>MLQVHRTGLGRLGVSLSKGLHHKAVLAVRREDVNAWERRAPLAPKHIKGITNLGYKVLIQPSNRRAIHDKDYVKAGGILQEDISEACLILGVKRPPEEKLMSRKTYAFFSHTIKAQEANMGLLDEILKQEIRLIDYEKMVDHRGVRVVAFGQWAGVAGMINILHGMGLRLLALGHHTPFMHIGMAHNYRNSSQAVQAVRDAGYEISLGLMPKSIGPLTFVFTGTGNVSKGAQAIFNELPCEYVEPHELKEVSQTGDLRKVYGTVLSRHHHLVRKTDAVYDPAEYDKHPERYISRFNTDIAPYTTCLINGIYWEQNTPRLLTRQDAQSLLAPGKFSPAGVEGCPALPHKLVAICDISADTGGSIEFM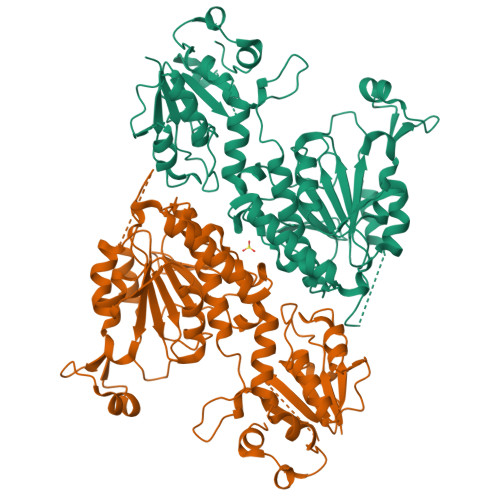TECTTIEHPFCMYDADQHIIHDSVEGSGILMCSIDNLPAQLPIEATECFGDMLYPYVEEMILSDATQPLESQNFSPVVRDAVITSNGTLPDKYKYIQTLRESRERAQSLS[4x]(5S)-5-methyl-5-[(1-phenyl-1H-1,2,3-triazol-4-yl)methyl]pyrrolidine-2,4-dione 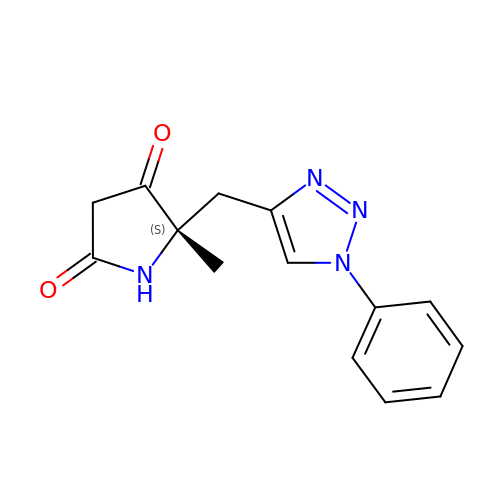| C14 H14 N4 O2 | JRHLMUQJOCQPQH-AWEZNQCLSA-N>[4x]MASEFKKKLFWRAVVAEFLATTLFVFISIGSALGFKYPVGNNQTAVQDNVKVSLAFGLSIATLAQSVGHISGAHLNPAVTLGLLLSCQISIFRALMYIIAQCVGAIVATAILSGITSSLTGNSLGRNDLADGVNSGQGLGIEIIGTLQLVLCVLATT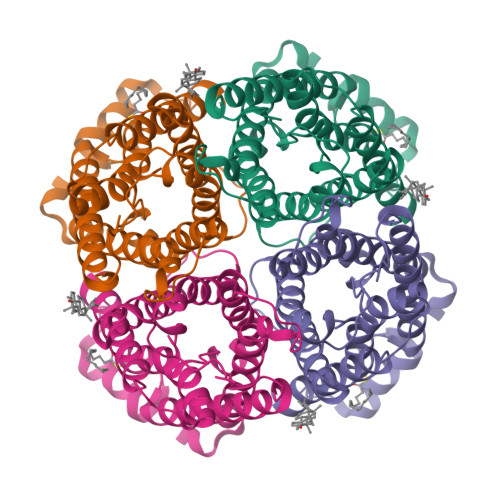DRRRRDLGGSAPLAIGLSVALGHLLAIDYTGCGINPARSFGSAVITHNFSNHWIFWVGPFIGGALAVLIYDFILAPRSSDLTDRVKVWTSGQVEEYDLDADDINSRVEMKPK> GSMESRKLISATDIQYSGSLLNSLNEQR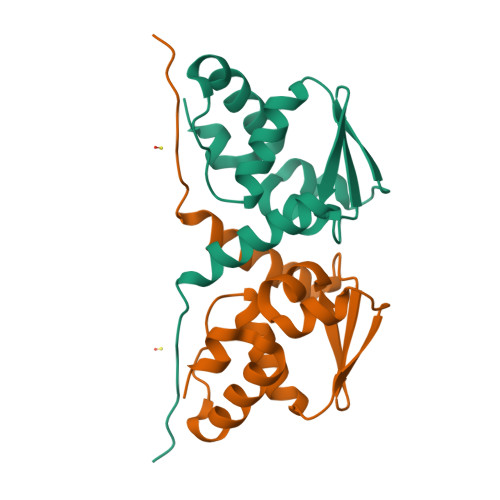GHGLFCDVTVIVEDRKFRAHKNILSASSTYFHQLFSVAGQVVELSFIRAEIFAEILNYIYSSKIVRVRSDLLDELIKSGQLLGVKFIAELGVPLSQ(3R)-1-[2-(4-methylphenyl)-2H-pyrazolo[3,4-d]pyrimidin-4-yl]-N-{[4-(methylsulfanyl)phenyl]methyl}piperidine-3-carboxamide 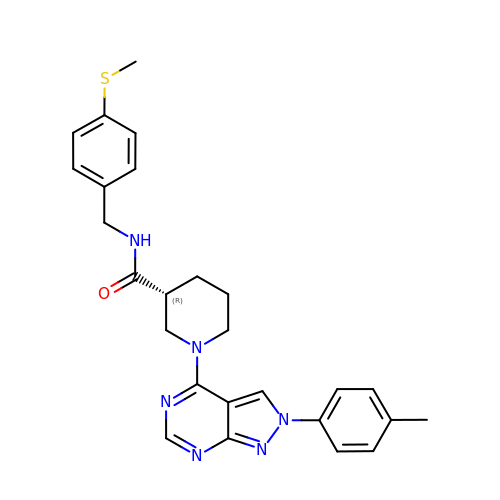| C26 H28 N6 O S | VWUOWUZLQDJSCV-HXUWFJFHSA-N> SELSFNYPNFQSVEDITFQGGASPRNETLQLTPTDSNGIPIRQRAGHAVYSQPFQLRDTSFYTTFTFVIRTTSNSPADGFAIFIAPPDFPVKRYGGYLGLFEPNTATNTSANKVVAVEFDTWVNTEWKEPRYRHIG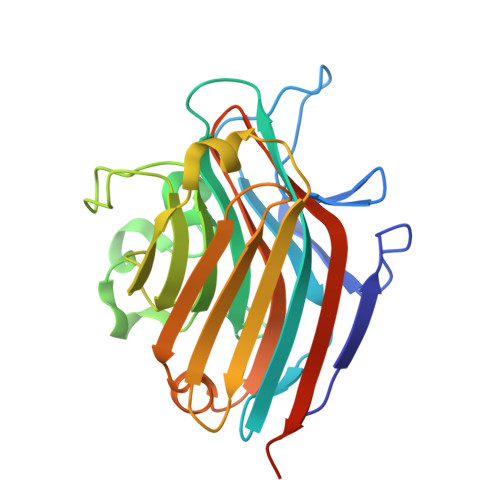IDVNSIVSVRVTRWQDKDVFSRSIATAHVGYDGISKILTAFVTYPDGGNYVLSHVVDLAEIFPGDVRIGFSGATGQYETQYIHSWSFSSTSTNLLRDGARHHHHHH> MQSKRGRPRNIETQKAILSASYELLLESGFKAVTVDKIAERAKVSKATIYKWWPNKAAVVMDGFLSAAAARLPVPDTGSALNDILIHATSLANFLISREGTIINELVGEGQ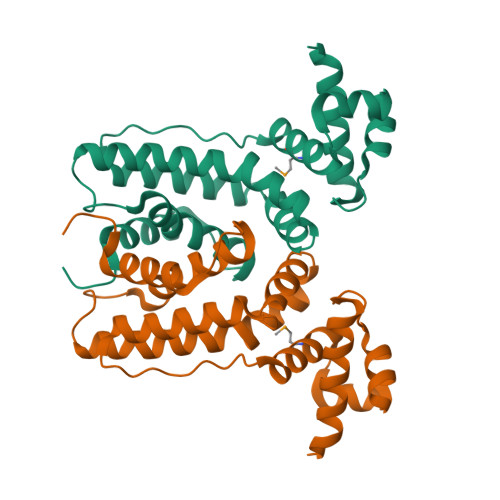FDSKLAEEYRVRYFQPRRLQAKQLLEKGIKRGELKENLDIELSIDLIYGPIFYRLLVTGEKLDDSYVHDLVINAFEGIRLR>MLTQTLKTQVINTQIGGKIAPPHQVSDQFGAITGHVGLVATEFSYRKDEEIYGEDEPAEYVYQVVTGAVRSYKLLSDGRRQIGAFHLPGDVFGLESGPSHRLAAEAIIDTSVRLVKRSSLEKAAGIDVQVAR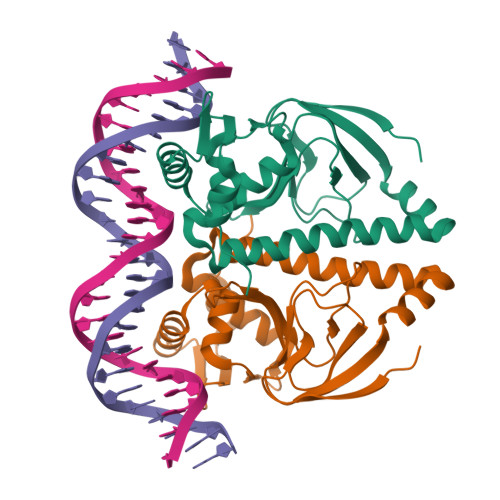KLWAMTAGELRHAEDHMLLLGRKTAMERVATFLLEMDRRLAVAGMMALPMSRRDIGDYLGLTLETVSRALSQLHTQGILGFSGARQIVLRNRQRLHNLDAAAALEHHHHHH[2x]>MAVELGVLLVRPRPGTGLGRVMRTLLLVLWLATRGSALYFHIGETEKKCFIEEIPDETMVIGNYRTQLYDKQREEYQPATPGLGMFVEVKDPEDKVILARQYGSEGRFTFTSHTPGEHQICLHSNSTKFSLFAGGMLRVHLDIQVGEHANDYAEIAAKDKLSELQLRVRQLVEQVEQIQKEQNYQRWREER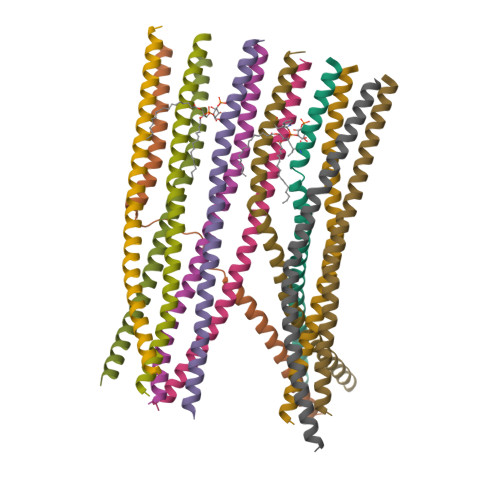FRQTSESTNQRVLWWSILQTLILVAIGVWQMRHLKSFFEAKKLV[12x]> SIVTKSIVNADAEARYLSPGELDRIKSFVLSGARRVRIAQTLTENRERIVKQAGDQLFQKRPDVVSPGGNAYGEEMTATCLRDLDYYLRLVTYGIVSGDVTPIEEIGLVG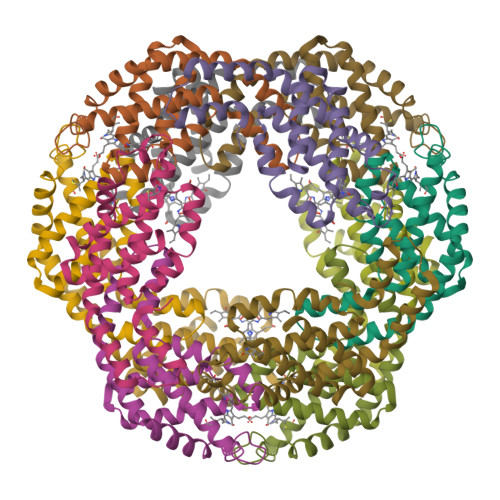VREMYKSLGTPISAVAEGVKCMKSVASSLLSGEDSAEAGFYFDYVVGAMQ;> MQDAITSVINSSDVQGKYLDSSAIEKLKGYFQTGELRVRAATTIAANAANIIKEAVAKSLLYSDITRPGGNMYTTRRYAACIRDLDYYLRYATYAMLAGDPSILDERVLNGLKETYNSLGVPIGATIQAIQAMKEVTSGLVGPDAGKEMGLYFDYICSGLS>AKVSLEKDKIKFLLVEGVHQKALESLRAAGYTNIEFHKGALDDEQLKESIRDAHFIGLRSRTHLTEDVINAAEKLVAIGCFCIGTNQVDLDAAAKRGIPVFNAPFSNTRSVAELVIGELLLLLRGVPEANAKAHRGVWNKLAAGSFEARGKKLGIIGYGHIGTQLGILAESLGMYVYFYDIENKLPLGNATQVQHLSDLLNMSDVVSLHVPENPSTKNMMGAKEISLMKPGSLLINASRGTVVDIPALCDALASKHLAGAAIDVFPTEPATNSDPFTSPLCEFDNVLLTPHIGGSTQEAQENIGLEVAGKLIKYSDNGSTLSAVNFPEVSLPLHGGRRLMHIHENRPGVLTALNKIFAEQGVNIAAQYLQ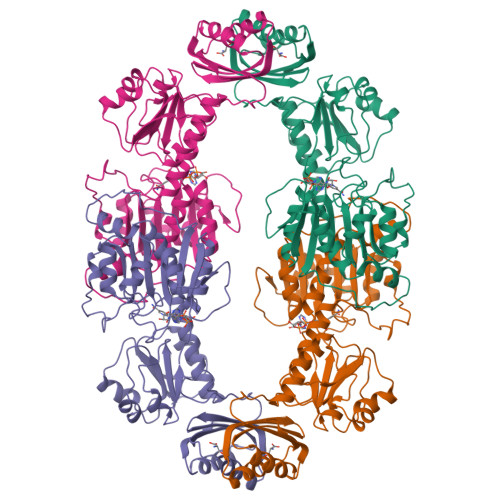TSAQMGYVVIDIEADEDVAEKALQAMKAIPGTIRARLLY[2x]> GVVDSCCRNSCSFSTLRAYC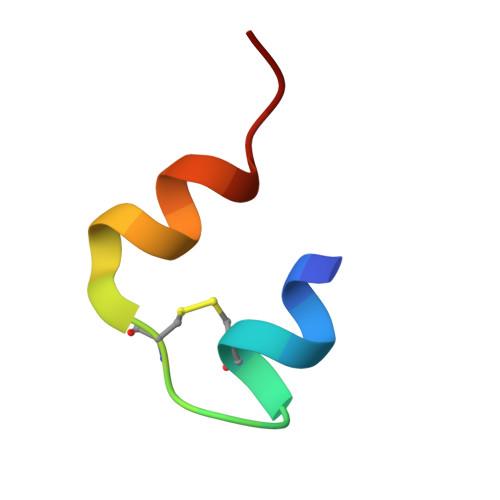DS>MVFPMWTLKRQILILFNIILISKLLGARWFPKTLPCDVTLDVPKNHVIVDCTDKHLTEIPGGIPTNTTNLTLTINHIPDISPASFHRLDHLVEIDFRCNCVPIPLGSKNNMCIKRLQIKPRSFSGLTYLKSLYLDGNQLLEIPQGLPPSLQLLSLEANNIFSIRKENLTELANIEILYLGQNCYYRNPCYVSYSIEKDAFLNLTKLKVLSLKDNNVTAVPTVLPSTLTELYLYNNMIAKIQEDDFNNLNQLQILDLSGNCPRCYNAPFPCAPCKNNSPLQIPVNAFDALTELKVLRLHSNSLQHVPPRWFKNINKLQELDLSQNFLAKEIGDAKFLHFLPSLIQLDLSFNFELQVYRASMNLSQAFSSLKSLKILRIRGYVFKELKSFNLSPLHNLQNLEVLDLGTNFIKIANLSMFKQFKRLKVIDLSVNKISPSGDSSEVGFCSNARTSVESYEPQVLEQLHYFRYDKYARSCRFKNKEASFMSVNESCYKYGQTLDLSKNSIFFVKSSDFQHLSFLKCLNLSGNLISQTLNGSEFQPLAELRYLDFSNNRLDLLHSTAFEELHKLEVLDISSNSHYFQSEGITHMLNFTKNLKVLQKLMMNDNDISSSTSRTMESESLRTLEFRGNHLDVLWREGDNRYLQLFKNLLKLEELDISKNSLSFLPSGVFDGMPPNLKNLSLAKNGLKSFSWKKLQCLKNLETLDLSHNQLTTVPERLSNCSRSLKNLILKNNQIRSLTKYFLQDAFQLRYLDLSSNKIQMIQKTSFPENVLNNLKMLLLHHNRFLCTCDAVWFVWWVNHTEVTIPYLATDVTCVGPGAHKGQSVISLDLYTCELDLTNLILFSLSISVSLFLMVMMTASHLYFWDVWYIYHFCKAKIKGYQRLISPDCCYDAFIVYDTKDPAVTEWVLAELVAKLEDPREKHFNLCLEERDWLPGQPVLENLSQSIQLSKKTVFVMTDKYAKTENFKIAFYLSHQRLMDEKVDVIILIFLEKPFQKSKFLQLRKRLCGSSVLEWPTNPQAHPYFWQCLKNALATDNHVAYSQVFKETV[2x];>[2x]MEAEPPLYPMAGAAGPQGDEDLLGVPDGPEAPLDELVGAYPNYNEEEEERRYYRRKRLGVLKNVLAASAGGMLTYGVYLGLLQMQLILHYDETYREVKYGNMGLPDIDSKMLMGINVTPIAALLYTPVLIRFFGTKWMMFLAVGIYALFVSTNYWERYYTLVPSAVALGMAIVPLWASMGNYITRMAQKYHEYSHYKEQDGQGMKQRPPRGSHAPYLLVFQAIFYSFFHLSFACAQLPMIYFLNHYLYDLNHTLYNVQSCGTNSHGILSGFNKTVLRTLPRSGNLIVVESVLMAVAFLAMLLVLGLCGAAYRPTEEIDLRSVGWGNIFQLPFKHVRDYRLRHLVPFFIYSGFEVLFACTGIALGYGVCSVGLERLAYLLVAYSLGASAASLLGLLGLWLPRPVPLVAGAGVHLLLTFILFFWAPVPRVLQHSWILYVAAALWGVGSALNKTGL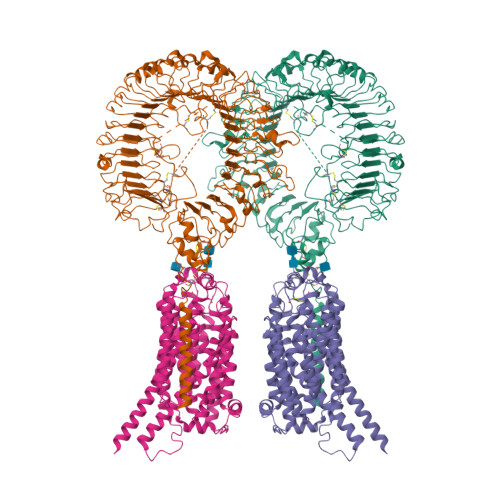STLLGILYEDKERQDFIFTIYHWWQAVAIFTVYLGSSLHMKAKLAVLLVTLVAAAVSYLRMEQKLRRGVAPRQPRIPRPQHKVRGYRYLEEDNSDESDAEGEHGDGAEEEAPPAGPRPGPEPAGLGRRPCPYEQAQGGDGPEEQ>GIRMDDSEDTSWDFGPQAFKLLSAVDILGEKFGIGLPILFLRGSNSQRLADQYRRHSLFGTGKDQTESWWKAFSRQLITEG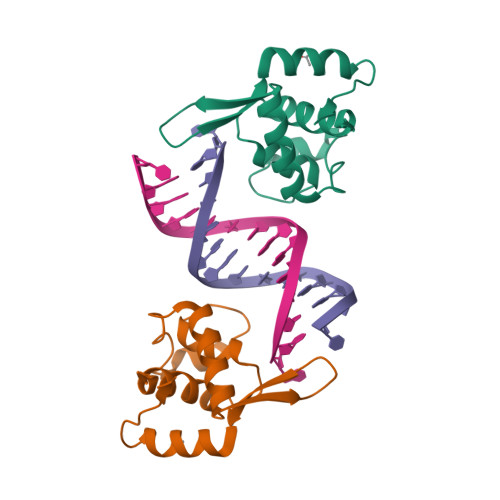FLVEVSRYNKFMKICALTKKGRNWLHKANTESQSLILQANEELCPKKFLLPSS[2x]> MVHHHHHHVIDLLQADGNALPSAVKLAYSPASKTFESYRV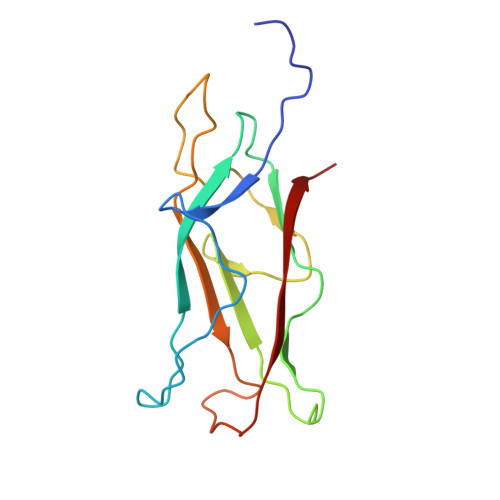MTQVHTNADAKKVIVKLADTPQATDVLNSTVQMPISVSWGGQVLSTTAKEFEAAALGYSASGVNGVSSSQELVISAAPKTAGTAPTAGNYSGVVSLVMTLGS(2R,3S)-4-(4-chlorophenyl)-2-phenyl-3-(1H-1,2,4-triazol-1-yl)butan-2-ol 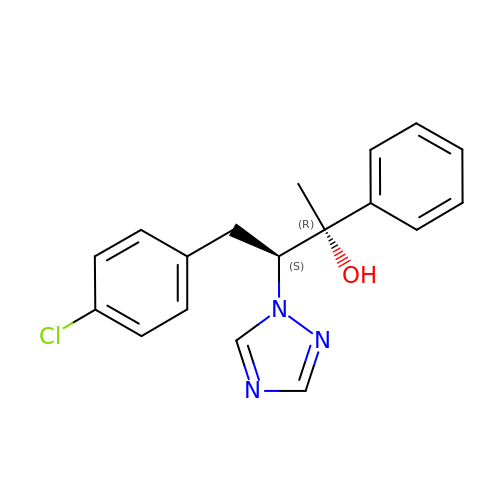| C18 H18 Cl N3 O | YULDTPKHZNKFEY-ZWKOTPCHSA-N> NLYQFKNMIQCTVPSRSWWDFADYGCYCGRGGSGTPVDDLDRCCQVHDNCYNEAEKISGCWPY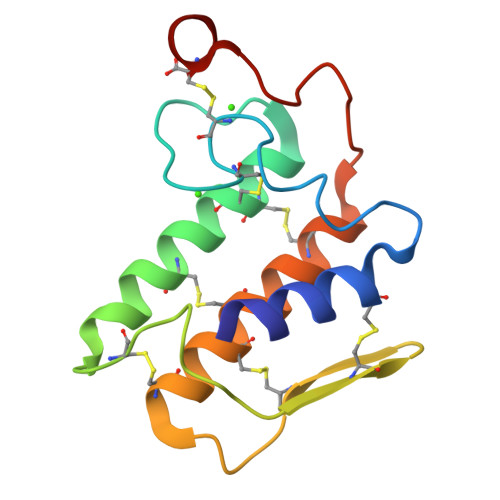FKTYSYECSQGTLTCKGGNNACAAAVCDCDRLAAICFAGAPYNDNDYNINLKARC>[3x]MIIDCHGHVSAPVELWAYKASLLAHRGSHGRGGVKVTDEQIIAAAHHKETWPDGHIELLHNHGTDMQLISPRPFQMMNSAKPARVVHWFCEEVNTLIHRQCTLIPEMFIPVAGLPQVAGEPIENVFAEMDRCVSMGFKGFLLNPDPYENGAEEAPPLGDRYWYPLYEKLC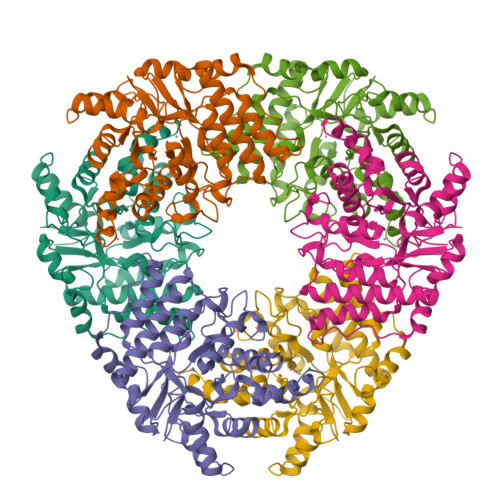ELDLPAHIHATGSQSERSPYSLHFINEETIATYNLCTSSVFDDFPQLKVVVSHGGGAIPYQLGRFESQSRRSKHLFSERMAKLYFDTVLYTEGALRLLIETVGPERCLFGSECPGVGSTIDPATGKQMDHIAPFIQKFDFLSDADKKLIFEDNARKVFNLEVENLYFQ>MECLRSLPCLLPRAMRLPRRTLCALALDVTSVGPPVAACGRRANLIGRSRAAQLCGPDRLRVAGEVHRFRTSDVSQATLASVAPVFTVTKFDKQGNVTSFERKKTELYQELGLQARDLRFQHVMSITVRNNRIIMRMEYLKAVITPECLLILDYRNLNLEQWLFRELPSQLSGEGQLVTYPLPFEFRAIEALLQYWINTLQGKLSILQPLILETLDALVDPKHSSVDRSKLHILLQNGKSLSELETDIKIFKESILEILDEEELLEELCVSKWSDPQVFEKSSAGIDHAEEMELLLENYYRLADDLSNAARELRVLIDDSQSIIFINLDSHRNVMMRLNLQLTMGTFSLSLFGLMGVAFGMNLESSLEEDHRIFWLITGIMFMGSGLIWRRLLSFLGRQLEAPLPPMMASLPKKTLLADRSMELKNSLRLDGLGSGRSILTNRDYKDDDDK[5x]

Most of the Mg2+ influx into mitochondria is mediated by the Mitochondrial RNA Splicing 2 (MRS2) channel, located in the inner mitochondrial membrane. MRS2 belongs to the CorA protein superfamily characterized by a highly conserved Glycine-Methionine-Asparagine (GMN) motif in the loop between transmembrane helix 1 and 2. MRS2 assembles into a homo-pentamer and displays an overall architecture similar to structures in the CorA family, with slight differences in the secondary structure arrangement. Along the pore, R332 and M336 have been identified as the main gating residues.

To investigate whether MRS2 undergoes conformational changes in response to environmental Mg2+ concentrations, we depleted most of the free Mg2+ in purified MRS2 using dialysis and addition of EDTA and performed structural analysis by cryo-EM. The resulting structures of MRS2 in the presence of 1 mM EDTA (referred to as MRS2-EDTA) with C5 symmetry and without symmetry applied (C1) were determined at an average resolution of 3.3 Å and 3.6 Å, respectively, with the highest local resolution estimated to be 2.7 Å. Unlike TmCorA, no significant structural changes can be observed when EDTA was included in the sample buffer. The Cα RMSD between MRS2-Mg2+ and MRS2-EDTA is 0.481 Å. In the central pore regions, densities for Mg2+−1, 2, 3 but not for Mg2+-4 were observed along the pore of MRS2 even after dialysis and addition of EDTA which should remove most of the free Mg2+ in the solution. The GMN motif is known to have a high affinity towards Mg2+ with an estimated KD of 1.3 µM36, which may be able to trap Mg2+ in the pore in the presence of EDTA. The conservation of Mg2+−1, 2, 3 and the loss of Mg2+-4, which is just below the R332/M336-rings, further suggests the gating properties of these residues and that MRS2 remains at low channel open probability without activation. While inspecting the Mg2+-binding sites found in the HsMRS2 structure in the presence of Mg2+, we do observe scattered densities in soluble site 2 but not soluble site 1. However, due to (1) the lower overall and local resolution of the MRS2-EDTA structure and (2) under EDTA conditions Mg2+ is not expected to be found in the position that is exposed to solvent, we speculate that these extra densities may represent water molecules coordinated by surrounding negatively charged residues. We have not modeled anything into these extra densities due to the high uncertainty.> MAQWVPKTAWKVSNLNKRYGPGYITSGFSSENTLGYTHMVHDSHKLREKLSSRKGIFVIDVRDPGERKLNPVP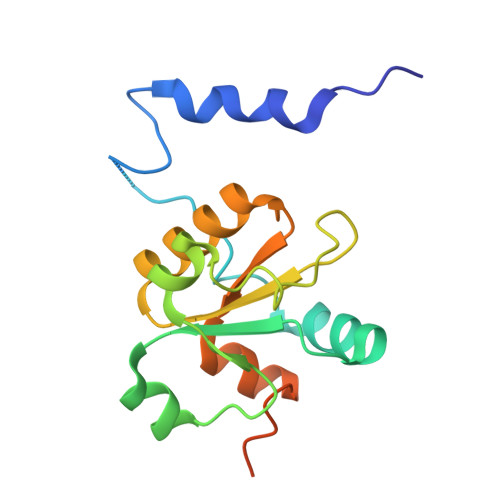RSVALHHHDLLSGASCPILPQQKSAAELFVLASNESRGLNSAAALRRWGYDSVVQVDYNTLVEAGYVSRCDYATAGTKDSAEQAVSGED>[2x]GSRADFFTYETTKSVVVKSWTIGIINRVVQLLIISYFVGWVFLHEKAYQVRDTAIESSVVTKVKGSGLYANRVMDVSDYVTPPQGTSVFVIITKMIVTENQMQGFCPESEEKYRCVSDSQCGPERLPGGGILTGRCVNYSSVLRTCEIQGWCPTEVDTVETPIMMEAENFTIFIKNSIRFPLFNFEKGNLLPNLTARDMKTCRFHPDK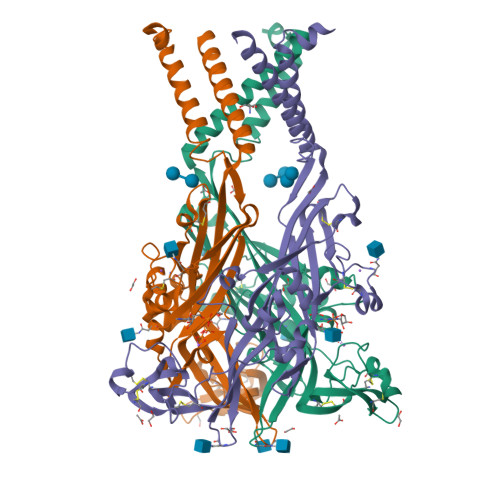DPFCPILRVGDVVKFAGQDFAKLARTGGVLGIKIGWVCDLDKAWDQCIPKYSFTRLDSVSEKSSVSPGYNFRFAKYYKMENGSEYRTLLKAFGIRFDVLVYGNAGKFNIIPTIISSVAAFTSVGVGTVLCDIILLNFLKGADQYKAKKFEEVNET>[8x]GSMTPRKVARILVAPNERDAAR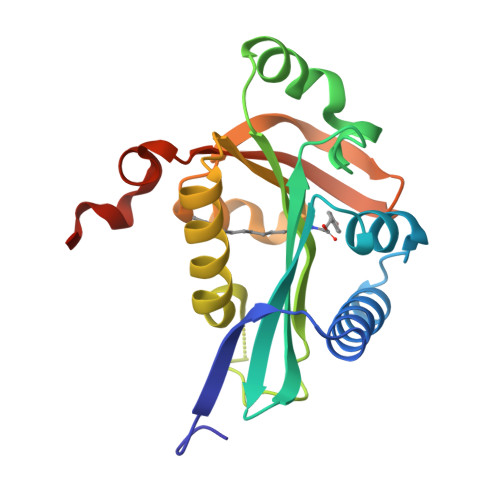RIVRTTYEAQGYAIDESFATFLEGPSATTFGLFNGEVLYGTISIINDGAQGLPMDSIYAVELAAWRGEGKKLAEVVQFAMDHTLYEAVAGAKPSPFEAASLFTMVLTYALETHIDYLCISINPKHDTFYSLLGFTQIGALKHYGTVNAPAIARALYVPEWRSQTLLAQFMDAERSH> MIRGSSALKSLTSRRLYSTGVKYTTLSNGVTVATETNPAAKTSSVGLFFGAGSRSEHSHSNGISALTTNVLASQSAKGSLLTAKNDREFNGIIAQTTNDNITEAGKLIASIASNAVDIVEKTDLTKHKQYLSAQASAVEADPKSKVLSHLYSSAFQGYSLALPTLGTTESVENLENQDSLRHLAKHLVNNNTVIAASGNFDHDKLADAIEANLKIAEGVKPEIKPASFLGSEVRMRDDTLPKAYISIAVHGEGLNSPNYYLAKVAAAIYGDFYLHSTIAKFTSPKLASIVQEYNIVESYNHYSKSFSDTGIWGYYAEIADKFTVDDFTHFSLKEWNRLSISISEAEVARAKAQVKTALAKELANSFAVTSDIAEKVLLVGHRQSLREAFEKIDAIKVNDVKEWGKSKVWDRDIVISGTGLIEDLLDYNRNRNEMAMMRW;> MLSR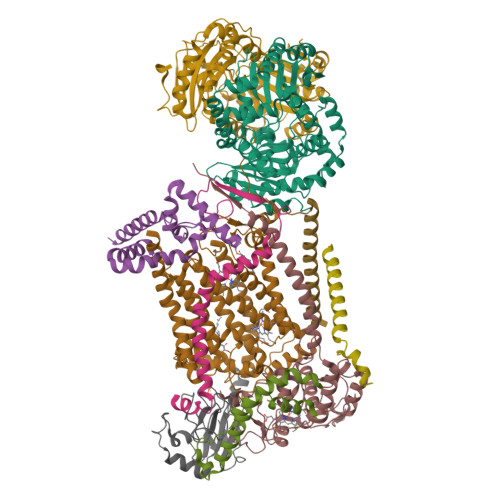ASIRAYSSIPNSVKIAAKESATDLTKLSVIINNAGSKTGKSGVSHLLSKFTFLNNGAKSALRFTRESELLGGTFESKVTRDALILNTTFLKQDLPYYVEALGNVVSNTQFAPHEFNEIVLPTANAETKLANANPAFKGVEKLHEITFRRGLGNPLFYNESTPIKLEEVAQFSKEQFSGENISIVAEGANEEDLTKFVSESAFCYLPSSSSNGAKALPTNTFTGQEARVPSSGASSALIGIPVKPADFGKYEVLSAAIGTSTLPSTSTPLAQIPGATSHLYKYQDAGLFVISVSGEASQVAQGIKQAKSVAESVSSSALSEAVKAAELSVALQSTVDSPLNVKVVAEEAPISKFNYVAVGDLDVLPYADEL;> MFRTAYKTMNQSMVQKFIAGGVGVTGLTASYLLYQDSMTADAMTAAEHGLHPPAYNWPHNGMFETFDHASIRRGFQVYREVCAACHSLDRIAWRNLVGVSHTTSEAKAMAEELEYDDEPDDEGKPRKRPGKLADYIPGPYENEQAARAANQGAYPPDLSLIVKARHGGSDYIFSLLTGYPDEPPAGVVLPEGSNYNPYFPGGAIAMGRVLFDDLVEYEDGTPATTSQMAKDVSTFLNWASEPEHDDRKKWGLKALVVLSSLYLLSIWVKRFKWTPIKNRKFRFDPPKK;>MSSLAFRTLRNGLGLKSSVRALSTTTTTLSNYQQPDYSSYLNNKSGQGSRNFTYFMVGSMGLLSAAGAKSTVEAFLSSFAASADVLAMAKVEVKLGAIPEGKNVIIKWQGKPVFIRHRTADEIEEANQVDIKTLRDPQNDADRVKKPEWLIMLGICTHLGCVPIGEAGDFGGWFCPCHGSHYDISGRIRKGPAPLNLEIPEYDFTDDETLLVG[2x];> MAGAPHPHTYMGWWGSLGSPKQKYITQYTISPYAAKPLKGAAYNAVFNTFRRTKNQFLYVAIPFVVVWSIWTRARDYNEYLYTKEGREELERVNV;> MVQSMTSVVKAANFILARPTLSKIITPLAQKFTAYAGYREMGLKFNDLLLEETPIMQTAIKRLPSELNYSRNFRILTAHQLALSHQLLPAEKAVKPEEDDNYLIPYILEAEKEAFEKAELDNIEVKA;> MSFFRDLLESVVPTAYAEEPVEDVEVEQPEDAPEEEVSEETVEEEEEDDEDDDEDDEEEEETADPLDTLREECTKTAACKPFDHHFHECIERVTKEQEEPDYEHKHYKEDCIEEFFHLQHCVNDCVAPRLFNRLK;> ATIFGGAFAFQGFFDVAVNKWWEEHNKAKLWKNVKGKFL;> MPTRKSNTYLSLVNSYLIDSPQPSSINYWWNLGSLLGLCLVIQIASGVFLAMHYSSNIELAFDSVEHIMRDVNAGWLIRYIHANGASFFFICMYLHIGKALYYGSYKQPRVMLWVIGVVIFILTMAIAFMGYCLVYGQMSHWGATVITNLLSAIPFIGNDIVPFIWGGFSVSNPTIQRFFALHFLLPFILAALVCMHLMALHVHGSSNPVGITGNIDRLPMHPYFIFKDLITVFVFLLIFSLFVFYSPNTLGHPDNYIPGNPMVTPPSIVPEWYLLPFYAILRSIPDKLGGVIAMFGAILILLSLPYTDRSIIRGNSFKVLSKLAFYLFVFNFILLGNLGQLHVEVPYIQLGQFATAYYFAHYIIVVPVISTLENILYYIGTQTRVK(2S)-2-(4-chlorophenyl)-1-{4-[(5R,7R)-7-hydroxy-5-methyl-6,7-dihydro-5H-cyclopenta[d]pyrimidin-4-yl]piperazin-1-yl}-3-(propan-2-ylamino)propan-1-one 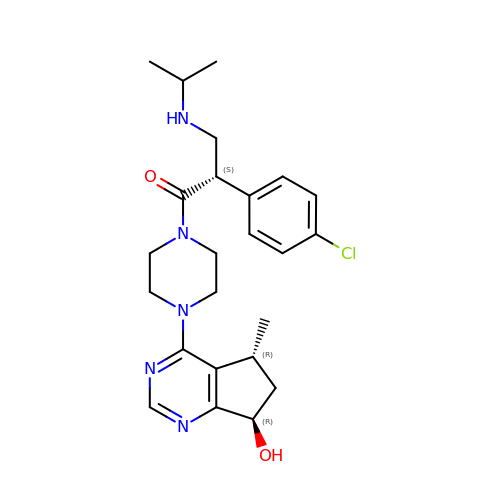| C24 H32 Cl N5 O2 | GRZXWCHAXNAUHY-NSISKUIASA-N> VMGEDQQIPRNEAQHGVHPISIDTHRISNNWSPQAMCIGEKVVSIRQLIKRFGIFGDANTLQADGSSFVVAPFTVTSPTKTLTSTRNYTQFDYYYYLYAFWRGSMRIKMV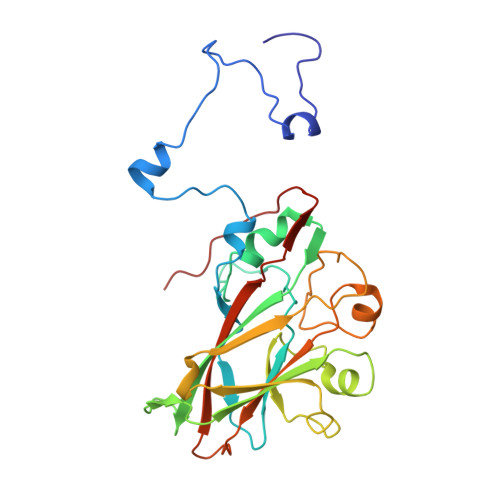AETQDGTGTPRKKTNFTWFVRMFNSLQDSFNSLISTSSSAVTTTVLPSGTINMGPSTQVIDPTVEGLIEVEVPYYNISHITPAVTIDDGTPSMEDYLKGHSPPCLLTFSPRDSISATNHIITASFMRALGDDFSFMYLLGVPPLVNVARA>[2x]GSDSSVNVALQASFDAGPYLLELLEAAAAENASSYFPLLDRIAEGVLDDAVTEKELYDRFLTIVQDEGHINDAADLSSFKFSLAIRSAVPRVEAHYQYYNTSVEPRLGTAQDAACPVWVHMDGMQYCSPTLERAQQAVSADLEARDLPFDRKLGDPTAPLAILYADVASPAFGEYHRKLSAMAKEGQVSYVVRYRPPPSASFRPLFLAGYGVELTLKRTDYIMIDDREAEESNEKQTNKRKVGSPSADELEEESPPDLKPLSSSEVARLGMNAASFILDSPDPFATLTKLSQDFPKYSSAVAAYNVTQEFLDEYYANRAASLPGGRNVLWINGLQIDSRQVDAYSLLEHLRHERQFIGQFRKLGLSNIEALDLLLHPNLTDGQSDAETQRYDWRDEVEGGDVIIWLNDLTKDKRYSDFPSDIDALLQPTYPGQLPAVRRDVHNVVIPIDLTNEDDVYMVVQHIQTFIKRLIPVRFGLVPLVHSEPAKSQAKIARYLQMTHGLAAMMKYFQRALEKDKLARPDQALFDETIASARVLRGKAQSFEEALSSTTLEEVMDKTGRYIKRLDLGGRSPPVLANGVLLGRGDNFLQELSMRVAIDLQLIQQSIVQDAVEEDTWLPSYFLSQAALTRNELIMPQDPSKIRIVNLVQVAESHDLTSLLRISAEGPGTNSLLMAVVGDFDSEAGLNLLISALKFRLAHPEIEVVPLHTSDDETNTHVSSQLYQLLRTERVDASEILEKIQIIKSTSDIGATATSKELAYWAQTKQLAADLGYPSGTRGVLLNGRAVGPVPSTSTLAEDDLEILLAYEFSKRLGTVAKVMKDLNLGHKVAGSVEFAKLTSLVALSTTSDIPEGIFESRSKYRQSAIKTWNGAHSAITVSHSDDASINIVATIDPASERSQRWVPILRTLSKLNGVNVKIFLTPVRILQELPIKRFYRHVLEPEPSFDEHGALNRPGASFSRLPEDALLTLGMDVPPSWLVSPKESVHDLDNIRLSSLREGSDVDAIYELEHILIEGHSTDVTTRSAPRGVQLLLGTDKNPHFADTIVMANLGYFQFKARPGFWKINLKPGPSQRIFNLDSVGGMGYQPKPGDETNEVALTSFQGRTLFPRLSRKPGHEEDDVLETGPKPG

Remarkably, the quality control system is equipped with an elaborate backup mechanism employing a molecular ‘gatekeeper’ that can specifically catalyse reglucosylation against incompletely folded glycoproteins as potential substrates, thereby regenerating monoglucosylated glycoforms for their return to the chaperone-assisted folding process. This gatekeeper function is executed by a unique enzyme, UDP-glucose:glycoprotein glucosyltransferase (UGGT). Our results reveal that UGGT has a modular structure in which the 35-kDa catalytic domain is tethered to the 125-kDa folding-sensor region. The N-terminal folding-sensor region is composed of the four Trx-like domains and the β-domain assembled into the C-shaped structure with structural plasticity harbouring the central cavity displaying hydrophobic patches, which putatively accommodates incompletely folded glycoproteins.

We determined the crystal structure of the N-terminal folding-sensor region of UGGT (UGGTN, residues 29–1142) at a 3.1-Å resolution. The overall structure of UGGTN displayed a C-shaped structure containing a large central cavity with 60 × 80 × 120 Å dimensions. The N-terminal Trx1 domain showed a unique Trx-like fold in which the four-helix subdomain was not inserted between β3 and β4 but preceded the α1-helix. In contrast, Trx2 and Trx3 domains exhibited a typical Trx-like fold comprising a four- or three-stranded β-sheet surrounded by six α-helices, in which the four-helix subdomain was inserted between β3 and β4. In the present T. dupontii UGGTN structure, the α6-helix was ordered in the detergent-free condition. The Trx4 domain represented a typical Trx-like fold comprising a four-stranded β-sheet surrounded by six α-helices, which, however, exhibited an unusual topology. Namely, in the four-helix subdomain, one core α-helix and β-strand are encoded by the N-terminal segment (residues 275–410), while three core β-strands and α-helix are encoded by the C-terminal segment (residues 897–950). Such uncommon domain architecture was also observed in the β-rich domain comprising six-stranded β-strands, which are encoded by three discrete segments (residues 29–39, 231–244 and 959–1036). Although we hypothesised that UGGT possesses a β-strand-rich domain comprising residues 942–1149 based on the bioinformatic analysis, only the N-terminal subdomain comprising residues 959–1036 gave unambiguous electron density, suggesting motional freedom in this domain. In the central cavity of the UGGTN C-shaped structure, remarkable hydrophobic patches were found, suggesting their possible involvement in folding-sensor function.>[2x]GGGTPKAPNLEPPLPEEE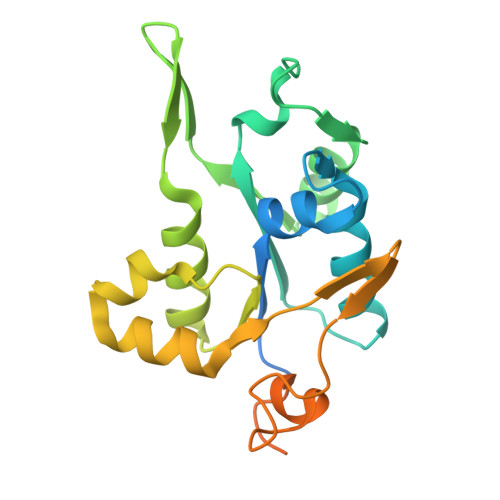KEGSDLRPVVIDGSNVAMSHGNKEVFSCRGILLAVNWFLERGHTDITVFVPSWRKEQPRPDVPITDQHILRELEKKKILVFTPSRRVGGKRVVCYDDRFIVKLAYESDGIVVSNDTYRDLQGERQEWKRFIEERLLMYSFVNDKFMPPDDPLGRHGPSLDNFLRKKPLTLEHRKQPCPYGRKCTYGIKCRFFHPERPSCPQRSVA MODIFIED ACARBOSE PENTASACCHARIDE | C31 H53 N O22 | 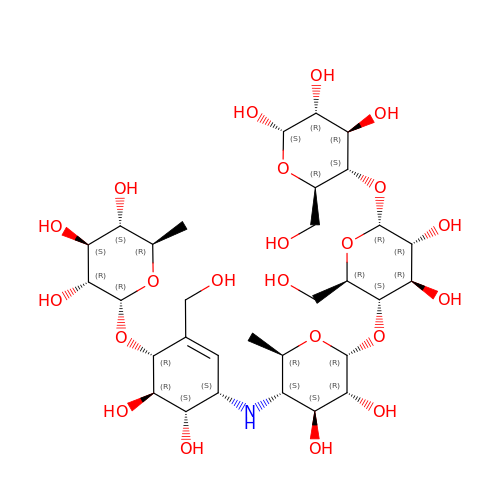QWNATFSCUHKKDP-WYKVUHPSSA-N>MTIKWIDWVKQIQSIAQAGLTYSKDVYDIERFQQLRDISISMMSHYTKTDWEVVEKLFASETGYQTPKVDIRAVVFQNEKLLFVKEKSDGKWALPGGWADVGYTPTEVAAKEVFEETGYEVDHFKLLAIFDKEKHQPSPSATHVYKIFIGCEIIGGEKKTSIETEEVEFFGENELPNLSIARNTEDQIKEMFAYMKDPQKE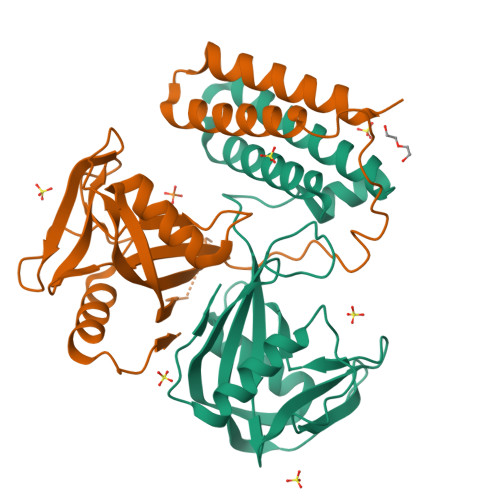KLID[2x]> XAVGPRGPSGPQGIRGDKGE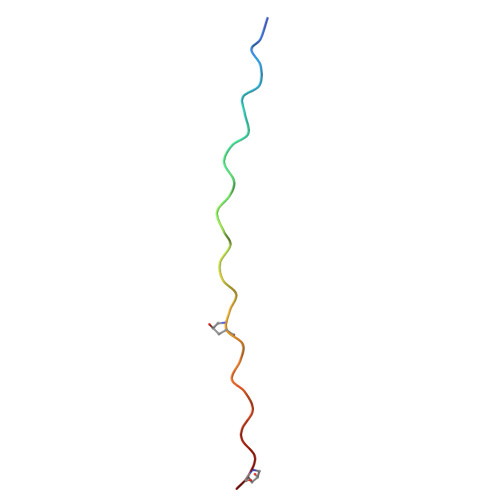PGEKGPRGLPG> GSHGNYAGNFSGSSRDICLDGARLRAECRRGDGGYSTSVIDLNRYLSNDNGHFRWVSTATVTV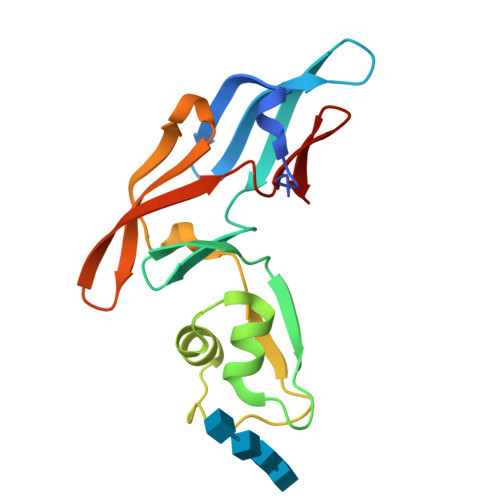QQGDTLRDIGRRFDCDFHEIARRNNIQNEDLIYPGQVLQVGGNFWDSARDVRLVDGGKVLEAELRYSGGWNRSRIYLDEHIGNRNGELIHC>NMSEVINFDQIFEGAIEPGKEPKRLFKEVYEGAITATSYAEILLSRAIEKYGPDHPVGYPDTAYFLPVIRAFSGEEVRTLKDMVPILNRMRAQIKSELTFENARLAGEATWYAAEIIEALRYLKHTPENPIVVPPWTGFIGDPVVRQYGIKMVDWTIPGEAIIIGRAKDSKAAKKIVDDLMGKGLMLFLCDEIIEQLLEENVKLGVDYIAYPLGNFTQVVHAANYALRAGLMFGGIAPGLRDAHRDYQRRRVLAFVLYLGEHDMVKTAAAMGAIFTGFPVITDQPLPEDKQIKDWFISEPDYDKIVQTALEVRGIKITSIDIDLPINFGPAFEGESIRKGDMHVEFGGGKTPSFELVRMVGPDEIEDGKVEVIGPDIDSVEPGGRLPIGIVVDIYGRKMQEDFEPVLERRIHYFTNYGEGFWHTAQRDLTWVRISKEAFAKGARLKHLGQLLYAKFKQEFPSIVDRVQVTIYTDEQKVLELREIARKKYAERDARLRELSDEAVDTYYSCLLCQSFAPTHVCIVSPERVGLCGAISWLDAKAAYEINPNGPNQPIPKEGLIDPVKGQWESFNEYIYKNSQRTIERMNLYTIMEYPMTSCGCFEAIMAYLPELNGFMIVNREHSGMTPIGMTFSTLAGMVGGGTQTPGFMGIGKSYIGSRKFVKAD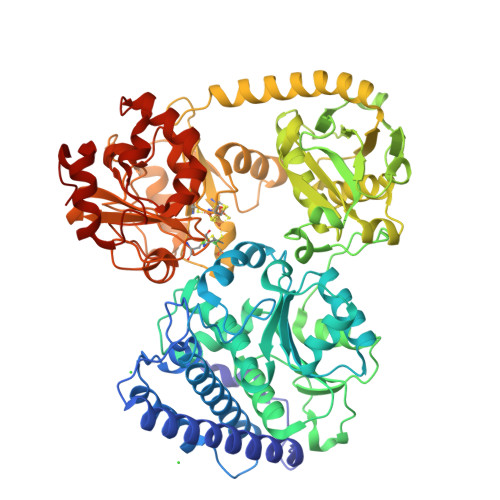GGLARVVWMPKDLKEQLRSIIEERAEEEGLGRDFIDKIADETVGTTVDEVLPFLEEKGHPALSMEPLL[2x]>SMFEIKKICCIGAGYVGGPTCSVIAHMCPEIRVTVVDVNESRINAWNSPTLPIYEPGLKEVVESCRGKNLFFSTNIDDAIKEADLVFISVNTPTKTYGMGKGRAADLKYIEACARRIVQNSNGYKIVTEKSTVPVRAAESIRRIFDANTKPNLNLQVLSNPEFLAEGTAIKDLKNPDRVLIGGDETPEGQRAVQALCAVYEHWVPREKILTTNTWSSELSKLAANAFLAQRISSINSISALCEATGADVEEVATAIGMDQRIGNKFLKASVGFGGSCFQKDVL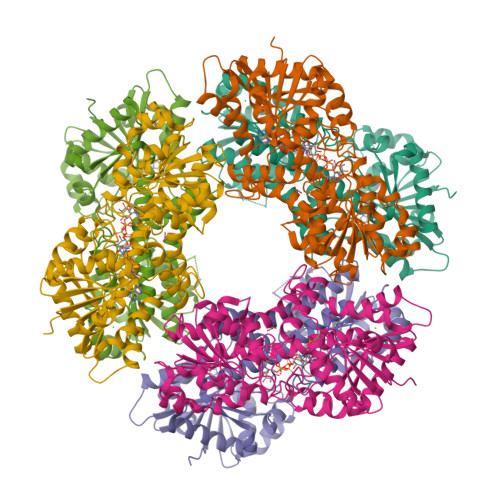NLVYLCEALNLPEVARYWQQVIDMNDYQRRRFASRIIDSLFNTVTDKKIAILGFAFKKDTGDTRESSSIYISKYLMDEGAHLHIYDPKVPREQIVVDLSHPGVSEDDQVSRLVTISKDPYEACDGAHAVVICTEWDMFKELDYERIHKKMLKPAFIFDGRRVLDGLHNELQTIGFQIETIGKKV[8x]>MSYQYVNVVTINKVAVIEFNYGRKLNALSKVFIDDLMQALSDLNRPEIRCIILRAPSGSKVFSAGHDIHELPSGGRDPLSYDDPLRQITRMIQKFPKPIISMVEGSVWGGAFEMIMSSDLIIAA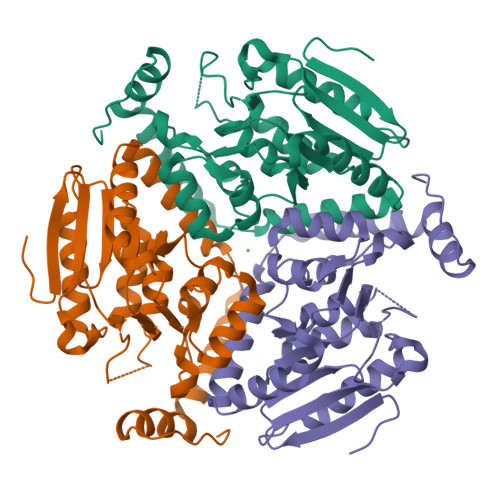STSTFSMTPVNLGVPYNLVGIHNLTRDAGFHIVKELIFTASPITAQRALAVGILNHVVEVEELEDFTLQMAHHISEKAPLAIAVIKEELRVLGEAHTMNSDEFERIQGMRRAVYDSEDYQEGMNAFLEKRKPNFVGH[3x]> MGIVGVGIDLVSIPDFAEQVDQPGTVFAETFTPGERRDASDKSSSAARHLAARWAAKEAVIKAWSGSRFAQRPVLPEDIHRDIEVVTDMWGRPRVRLTGAIAEYLADVTIHVSLTHEGD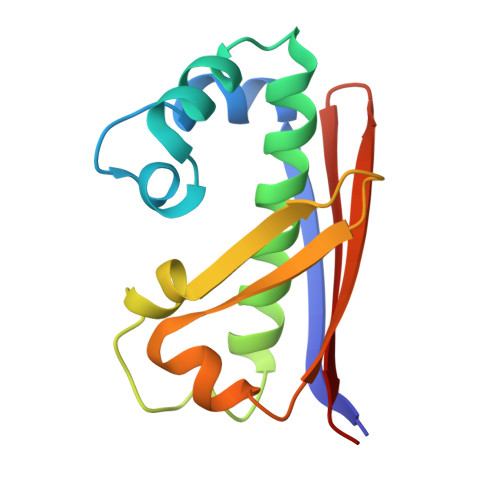TAAAVAILEAP> MAHHHHHHMLIPAEQLPPLKEEEVIEKIENDACIQK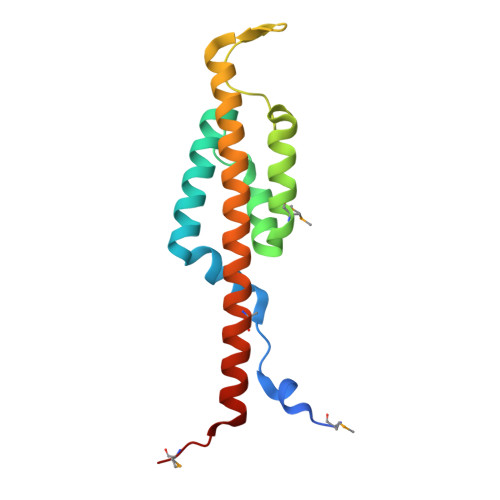SLEKIRALSKLIYNNPEILEQDISHINANPKMGRELSERIINSPKSIGRLKGRKIGYIKSQKYKISEQNAKILSNEIFNYADKVSNIRCTIMREHKAKGRRLLQTVKMPS> MGSSHHHHHHSSGLVPAGSHAGMIIDADYITEDGKPIIRIFKK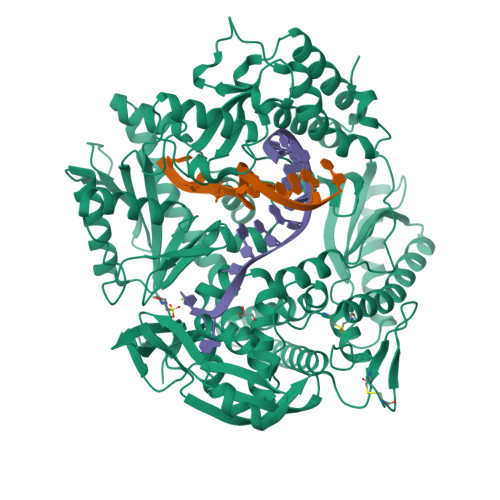EKGEFKVEYDRTFRPYIYALLKDDSAIDEVKKITAERHGKIVRITEVEKVQKKFLGRPIEVWKLYLEHPQDVPAIREKIREHPAVVDIFEYDIPFAKRYLIDKGLTPMEGNEELTFLAVDIETLYHEGEEFGKGPIIMISYADEEGAKVITWKSIDLPYVEVVSSEREMIKRLVKVIREKDPDVIITYNGDNFAFPYLLKRAEKLGIKLPLGRDNSEPKMQRMGDSLAVEIKGRIHFDLFPVIRRTINLPTYTLEAVYEAIFGKSKEKVYAHEIAEAWETGKGLERVAKYSMEDAKVTFELGKEFFPMEAQLARLVGQPVWDVSRSSTGNLVEWFLLRKAYERNELAPNKPDEREYERRLRESYEGGYVKEPEKGLWEGIVSLDFRSLYPSIIITHNVSPDTLNRENCKEYDVAPQVGHRFCKDFPGFIPSLLGNLLEERQKIKKRMKESKDPVEKKLLDYRQRAIKILANSYYGYYGYAKARWYCKECAESVTAWGRQYIDLVRRELESRGFKVLYIDTDGLYATIPGAKHEEIKEKALKFVEYINSKLPGLLELEYEGFYARGFFVTKKKYALIDEEGKIVTRGLEIVRRDWSEIAKETQAKVLEAILKHGNVDEAVKIVKEVTEKLSKYEIPPEKLVIYEQITRPLSEYKAIGPHVAVAKRLAAKGVKVKPGMVIGYIVLRGDGPISKRAIAIEEFDPKKHKYDAEYYIENQVLPAVERILRAFGYRKEDLKYQKTKQVGLGAWLKF The Hbl toxin is a three-component haemolytic complex produced by Bacillus cereus sensu lato strains and implicated as a cause of diarrhoea in B. cereus food poisoning. The toxin is composed of three components HblB, HblL1 and HblL2, all of which are essential for activity with no individual or pair wise activity. A crystal structure of the HblB component was published in 2008 and all components are predicted to share a similar fold, characteristic of the alpha pore-forming toxins (α‑PFTs), also related to the Nhe toxins of B. cereus (another 3-part toxin), the HlyE toxin from Escherichia coli and the App6 pesticidal protein from B. thuringiensis (known as Cry6 prior to a recent nomenclature revision). Although it has been reported that all components are able to bind to erythrocytes independently, more recent work strongly suggests that only the HblB component is able to bind and, thereby, to carry out a rate limiting priming step to allow lysis by the L components.

Here, we describe the expression of the recombinant HblL1 component and the elucidation of its structure to 1.36 Å. The electron density map showed continuous density for residues 41 to 404 (accession EEM59260.1) of the protein sequence. The overall fold comprises two almost parallel helical domains. Domain 1 is a bundle of five helices covering residues G41 to Q210 and R315 to K404. Domain 2 is a pair of two-helix bundles with an interleaving two strand β-sheet, covering the middle stretch of the sequence from residues A211 to D314. The points where the chain transitions between the two domains (residues 209–212 and 313–316) show some of the highest b factor scores in the structure and may represent hinge regions through which the two domains could move apart, although in the present structure they are in a closed conformation. Domain 2 in the head region also features the only beta hairpin in the structure, which is a typical feature of this class of protein, forming a hydrophobic beta tongue that has been shown in HlyE to undergo extensive structural rearrangement to contribute to the pore. In HblL1, however, this hydrophobic region is more extensive than in the other Hbl proteins, is rich in glycine and alanine residues and contains a central proline (Pro268) residue. No super structure or macro cluster of HblL1 is likely to exist in solution as a biological entity. In the computed complex, the beta tongue region of HblL1 is buried against the tail region of HblB; the β-tongue of HblB does not play a part in the dimer interaction.

> GNYALGPEGLKKALAETGSHILVMDLYAKTMIKQPNVNLSNIDLGSEGGELLKNIHLNQELSRINANYWLDTAKPQIQKTARNIVNYDEQFQNYYDTLVETVQKKDKAGLKEGINDLITTINTNSKEVTDVIKMLQDFKGKLYQNSTDFKNNVGGPDGKGGLTAILAGQQATIPQLQAEIEQLRSTQKKHFDDVLAWSIGGGLGAAILVIAAIGGAVVIVVTGGTATPAVVGGLSALGAAGIGLGTAAGVTASKHMDSYNEISNKIGELSMKADRANQAVLSLTNAKETLAYLYQTVDQAILSLTNIQKQWNTMGANYTDLLDNIDSMQDHKFSLIPDDLKAAKESWNDIHKDAEFISKDIAFKQ> GSE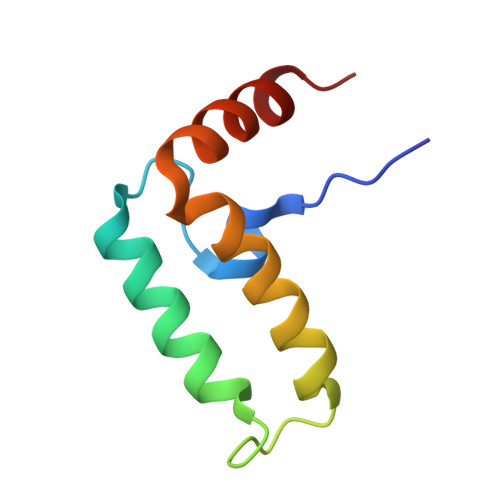LKDYYAIMGVKPTDDLKTIKTAYRRLARKYHPDVSKEPDAEARFKEVAEAWEVLSDEQRRAEYDQMWQHRN> MELTPREKDKLLLFTAALVAERRLARGLKLNYPESVALISAFIMEGARDGKSVASLMEEGRHVLTREQVMEGVPEMIPDIQVEATFPDGSKLVTVHNPII;> MIPGEYHVKPGQIALNTGRATCRVVVENHGDRPIQVGSHYHFAEVNPALKFDRQQAAGYRLNIPAGTAVRFEPGQKREVELVAFAGHRAVFGFRGEVMGPLEVNDE;> MSNISRQAYADMFGPTVGDKVRLADTELWIEVE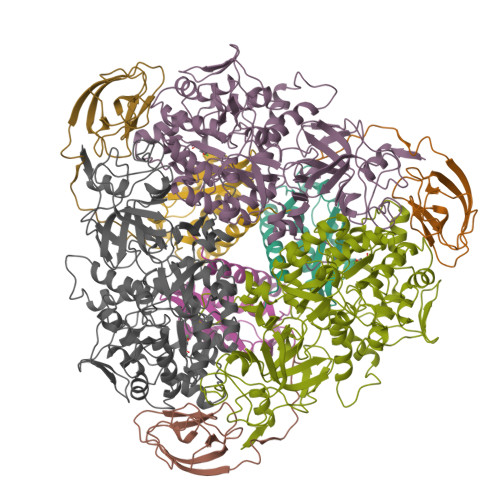DDLTTYGEEVKFGGGKVIRDGMGQGQMLAADCVDLVLTNALIVDHWGIVKADIGVKDGRIFAIGKAGNPDIQPNVTIPIGAATEVIAAEGKIVTAGGIDTHIHWICPQQAEEALVSGVTTMVGGGTGPAAGTHATTCTPGPWYISRMLQAADSLPVNIGLLGKGNVSQPDALREQVAAGVIGLKIAEDWGATPAAIDCALTVADEMDIQVALHSDTLNESGFVEDTLAAIGGRTIHTFHTEGAGGGHAPDIITACAHPNILPSSTNPTLPYTLNTIDEHLDMLMVCHHLDPDIAEDVAFAESRIRRETIAAEDVLHDLGAFSLTSSDSQAMGRVGEVILRTWQVAHRMKVQRGALAEETGDNDNFRVKRYIAKYTINPALTHGIAHEVGSIEVGKLADLVVWSPAFFGVKPATVIKGGMIAIAPMGDINASIPTPQPVHYRPMFGALGSARHHCRLTFLSQAAAANGVAERLNLRSAIAVVKGCRTVQKADMVHNSLQPNITVDAQTYEVRVDGELITSEPADVLPMAQRYFLF>GAMAMSDLPIEFTELVDLMSLGISPQFLDFRSTTFESDHFVTVRETKDGTNSVAIVDLAKGNEVTRKNMGGDSAIMHPSQMVISVRANGTIVQIFNLETKSKLKSFTLDEPVIFWRWLSETTLGFVTARSILTSNVFDGNVNAKPQLLTLRHANLNNTQIINFVANKNLDWFAVVGILQENGRIAGRIQLFSKQRNISQAIDGHVAIFTNILLEGNGSTPVQVFVTGNRNATTGAGELRIIEIDHDASLPSQYQKETTDIFFPPDATNDFPIAVQVSEKYGIIYLLTKYGFIHLYELETGTNLFVNRITA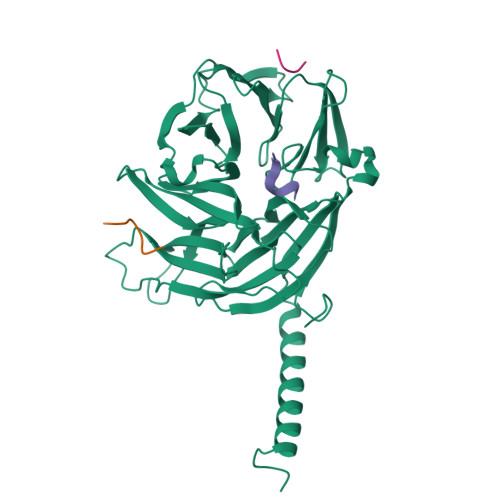ESVFTAAPYNHENGIACINKKGQVLAVEISTSQIVPYILNKLSNVALALIVATRGGLPGADDL[2x];>SQDLLDLF[5x]>[6x]MASVVPIAFDQVDNNTNATQLFKNNINKTRMNDLNREETR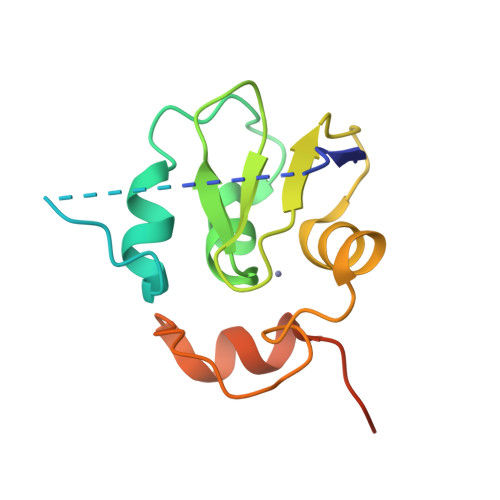LKTFTDWPLDWLDKRQLAQTGMYFTHAGDKVKCFFCGVEIGSWEQEDQPVPEHQRWSPNCPLLRRRTTNNVPINAEALDRILPPISYDLEHHHHHH>MADLAESNIKVMCRFRPLNESEVNRGDKYIAKFQGEDTVVIASKPYAFDRVFQSSTSQEQVYNDAAKKIVKDVLEGYNGTIFAYGQASSGKTHTMEGKLHDPEGMGIIPRIVQDIFNYIYSMDENLEFHIKVSYFEIYLDKIRDLLDVSKTNLSVHEDKNRVPYVKGATERFVSSPDEVMDTIDEGKSNRHVAVTNMNEHSSRSHSIFLINVKQENTQTEQKLSGKLYLVDLAGSEKVSKTGAEGAVLDEAKNINKSLSALGNVISALAEGSTYVPYRDSKMTRILQDSLGGNARTTIVICCSPSSYNESETKSTLLFGQRAKTI[6x]

Kinesins are a family of microtubule-based motors that play important roles in intracellular transport and cell division. Kinesin-1 transports cargo within cells, a process tightly coupled with ATP hydrolysis. Whereas kinesin-1 in solution is mostly loaded with ADP, ADP release is accelerated several thousand-fold upon microtubule binding. Here we characterized kinesin-1 P-loop mutations that interfere with ADP binding and determined the structure of the corresponding mutated nucleotide-free kinesins.

More importantly, when more mutations of residue 87 were tested, the T87A and T87G mutants were found to release ADP much faster than wild-type (koff = 2.77 s−1 and 4.80 s−1, respectively). Apo-T87A kinesin-1 was crystallized in a new crystal form following nucleotide digestion by apyrase and gel filtration to remove any trace of nucleotide. The crystals diffracted to 2.6 Å and there were six identical molecules in the asymmetric unit (r.m.s.d. of Cαs in pairs of molecules varies between 0.3 Å and 0.55 Å). The r.m.s.d. of Cαs of the apo-T87A kinesin-1 compared with ADP-kinesin-1 varies between 1.2 Å and 1.5 Å. By contrast, the conformation of apo-T87A is much more similar to that of apo wild-type kinesin-1 bound to tubulin, the r.m.s.d. of Cαs being close to 0.8 Å whatever the apo-T87A molecule considered. In contrast, apo-T87A differs from apo-kinesin-1 bound to tubulin in a small portion of the Switch 2 containing L11 loop: a stretch between Switch 2 and the α4 helix is disordered in apo-T87A whereas interactions with tubulin stabilize it in the complex. In apo-kinesin-1 bound to tubulin, the structure of L11 changes and E236 interacts with the Switch 1 residue R203. But in apo-T87A, where the structure of L11 has changed again, the R203-E236 interaction is lost and the E236 side-chain is disordered and not visible beyond Cβ. Since it is disordered in isolated T87A apo-kinesin-1, E236 does not make any visible interaction with the P-loop and with residue 87 in particular, leading to a higher mobility of the P-loop. P-loop destabilization, together with the removal of the nucleotide, leads to a tubulin-bound apo-kinesin-like conformation, as seen in the structure of the apo-T87A kinesin.>FSNLAIYWGQGPNQLRLSHFCQETSLDIINIGFINYFPDMSPGHWPGSNFGNQCDGSVYVTNDGVVTKLLSGCHQIMEDIPICQAAGKKVLLSIGGAYPPDQSILSEDSAVAFATFLWGAFGPVAEGWEGPRPFGDVVVDGFDFDIEHNGGFGYATMVNTFRQYFNQVPERKFYLSAAPQCIIPDAQLSDAIFNAAFDFIWIQYYNTAACSAKSFIDTSLGTFNFDAWVTVLKASASKDAKLYVGLPASETAANQGYYLTPDEVESLVSTYMDRYPDTFGGIMLWEATASENNQIDGAPYADHMKDILLH[2x]

A. fumigatus chitinase A1 (AfChiA1) also belongs to the class of plant-type chitinases family, and has been cloned and characterised recently. Because of the inherent rigidity of chitin, fungi need to partially hydrolyse the chitin layer for cell division and morphogenesis, which is carried out by family 18 chitinases. Whereas the ‘bacterial-type’ enzymes are invariably secreted and mostly possess exochitinase activity, the ‘plant-type’ chitinases are frequently cell wall associated and possess endochitinase activity. There are five ‘plant-type’ chitinases genes in the A. fumigatus genome (AfChiA1–5), with a currently unknown transcription profile.

AfChiA1 crystals, reported previously, were soaked with acetazolamide, diffraction data were collected to 2.0 Å resolution, and the structure of the AfChiA1–acetazolamide complex was solved by molecular replacement and refined to an Rfree of 0.249 with good stereochemistry. Electron density for the ligand acetazolamide can be seen in both molecules in the asymmetric unit, but it is less clear in chain A, where the active site is partially occluded by a symmetry-related protein molecule. Thus the further discussion of the structure will focus on chain B only, which is less impacted and has a more accessible active site. The overall binding mode of the ligand to AfChiA1 is essentially identical to that observed for ScCTS1. The thiadiazole ring stacks with the conserved Trp312, while its ring nitrogens accept hydrogen bonds from the backbone amides of Ala124 and Tyr125, in the latter case indirectly via an active site-bound water molecule. The acetamido group enters, and essentially fills, the small AfChiA1 active site pocket formed by Tyr238, Gln230, Met310, Ala205, Tyr34 and Asp172. It is oriented by two hydrogen bonds, one from its amide to the side chain of Asp172 and one from the Tyr232 side chain hydroxyl to its carbonyl oxygen. The sulfonamide group on the other hand forms few direct interactions with the protein: it accepts a poor hydrogen bond from the Trp312 side chain and otherwise points away from the protein and into the bulk solvent. Kinetin failed to show any discernable effect against AfChiA1 even at concentrations in excess of 1 mM; acetazolamide on the other hand inhibited AfChiA1 with an IC50 of 164 μM, which is an order of magnitude less potent than previously demonstrated against ScCTS1 but not dissimilar to the level of inhibition observed for allosamidin.>[6x]GSGSGSGMEKTQETVQRILLEPYKYLLQLPGKQVRTKLSQAFNHWLKVPEDKLQIIIEVTEMLHNASLLIDDIEDNSKLRRGFPVAH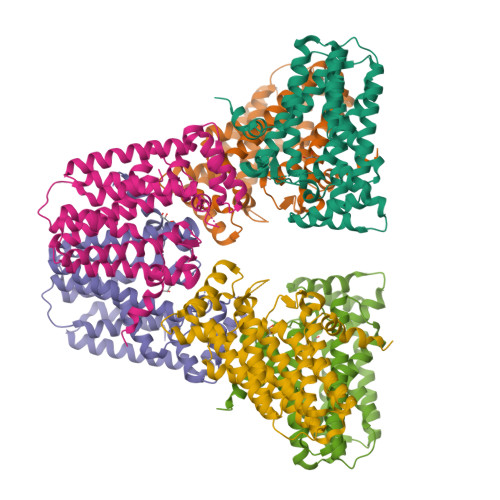SIYGIPSVINSANYVYFLGLEKVLTLDHQDAVKLFTRQLLELHQGQGLDIYWRDNYTCPTEEEYKAMVLQKTGGLFGLAVGLMQLFSDYKEDLKPLLNTLGLFFQIRYDYANLHSKEYSENKSFCEDLTEGKFSFPTIHAIWSRPESTQVQNILRQRTENIDIKKYCVHYLEDVGSFEYTRNTLKELEAKAYKQIDARGGNPELVALVKHLSKMFKEENE> MLTVIAEIRTRPGQHHRQA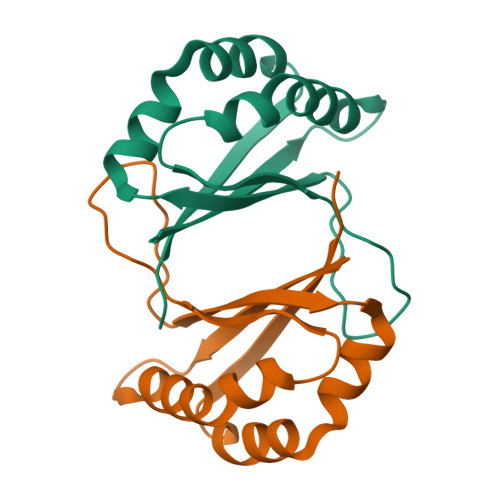VLDQFAKIVPTVLKEEGCHGYAPMVDCAAGVSFQSMAPDSIVMIEQWESIAHLEAHLQTPHMKAYSEAVKGDVLEMNIRILQPGISGRVEHHHHHH> SH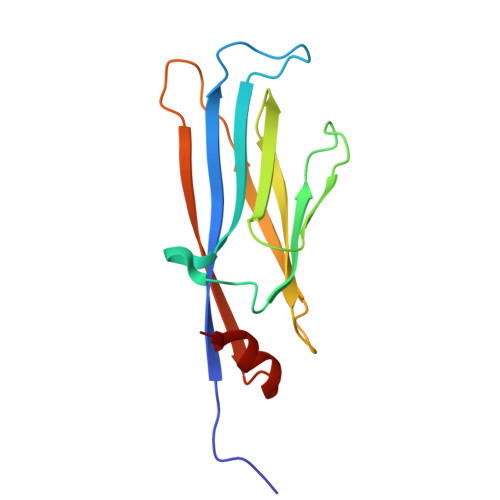MASSCAVQVKLELGHRAQVRKKPTVEGFTHDWMVFVRGPEHSNIQHFVEKVVFHLHESFPRPKRVCKDPPYKVEESGYAGFILPIEVYFKNKEEPRKVRFDYDLFLHLEGHPPVNHLRCEKLTFNNPTEDFRRKLLKA3-[(3~{S},4~{R})-4-azanyl-4-carboxy-1-[[(2~{S})-piperidin-2-yl]methyl]pyrrolidin-3-yl]propyl-tris(oxidanyl)boranuide | C14 H29 B N3 O5 | 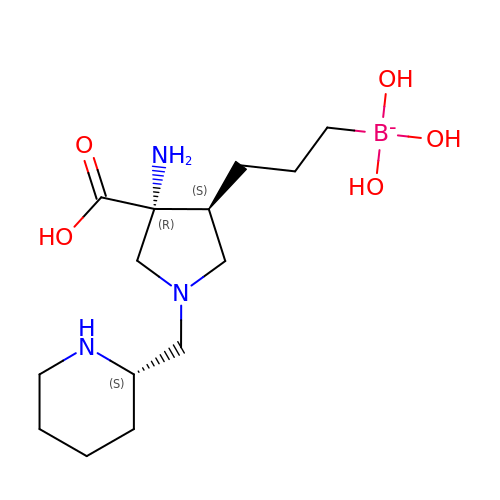UAQSNVVPOJZDTG-OBJOEFQTSA-N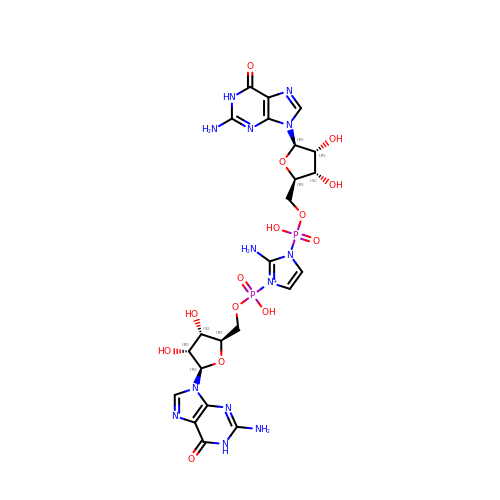2-amino-1-[(R)-{[(2R,3S,4R,5R)-5-(2-amino-6-oxo-1,6-dihydro-9H-purin-9-yl)-3,4-dihydroxyoxolan-2-yl]methoxy}(hydroxy)phosphoryl]-3-[(S)-{[(2R,3S,4R,5R)-5-(2-amino-6-oxo-1,6-dihydro-9H-purin-9-yl)-3,4-dihydroxyoxolan-2-yl]methoxy}(hydroxy)phosphoryl]-1H-imidazol-3-ium | C23 H30 N13 O14 P2 | NQKWYRRUFGLPHK-XPWFQUROSA-O The adhesin FimH at the fimbrial tip specifically binds in a catch-bond mode to terminal α-D-linked mannoses of N-linked glycans of the receptor uroplakin 1a on urinary epithelial cells. FimH is a two-domain protein, composed of an N-terminal, mannoside-binding lectin domain (FimHL) and a C-terminal pilin domain (FimHP). FimHP possesses an incomplete immunoglobulin-like fold that is completed by insertion of an N-terminal donor strand of FimG, the subsequent subunit in pilus assembly. The two-domain architecture of FimH is a prerequisite for catch-bond formation because the interactions between FimHL and FimHP determine the conformational state and ligand-binding properties of FimHL.

The crystal structure of the binary complex FimHF18·DsG was determined at atomic resolution by molecular replacement. FimHF18·DsG comprises the jellyroll fold FimHL and the immunoglobulin-like FimHP domain complemented with the FimG donor strand. It closely resembles unliganded FimH in the fimbrial tip complex, with a root-mean-square deviation of Cα positions (Cα r.m.s.d.) of 1.1 Å. The DsG peptide in FimHF18·DsG is in identical position as compared with the N-terminal FimG extension in the fimbrial tip structure; it interacts with β-strand 2 and 9 of FimHP. All contacts in the FimHL–FimHP interdomain region 17 as well as the conformation of the empty ligand-binding pocket observed in FimH in the fimbrial tip are preserved in FimHF18·DsG. Thus, FimHF18·DsG represents the ligand-free state of fimbrial FimH, with Associated FimHL and FimHP (Afree state) and is an elegant minimal system to analyse the crosstalk between ligand-binding and interdomain interactions underlying the formation of catch-bonds by FimH. In the absence of ligands, FimH adopts the Afree state with associated FimHL and FimHP and an open conformation of the ligand-binding site, which is responsible for the 30-fold faster ligand-binding of full-length FimH as compared with the isolated FimHL domain. The results revealed equilibrium dissociation constants (Kd) of 3.6 and 9.9 μM for FimHK12·DsG and FimHF18·DsG, respectively. The rates of HM dissociation (koff) of 22 and 58 s−1 for FimHK12·DsG and FimHF18·DsG translate into dissociation half-lives of only 32 and 12 ms, respectively.

> FACKTANGTAIPIGGGSANVYVNLAPAVNVGQNLVVDLSTQIFCHNDYPETITDYVTLQRGSAYGGVLSSFSGTVKYNGSSYPFPTTSETPRVVYNSRTDKPWPVALYLTPVSSAGGVAIKAGSLIAVLILRQTNNYNSDDFQFVWNIYANNDVVVPTGGCDVSARDVTVTLPDYPGSVPIPLTVYCAKSQNLGYYLSGTTADAGNSIFTNTASFSPAQGVGVQLTRNGTIIPANNTVSLGAVGTSAVSLGLTANYARTGGQVTAGNVQSIIGVTFVYQ;> ADVTITVNGKVVAK> GSSHHHHHHSQDLENLYFQGSWKLLPENGSGSSENSGFSGSQINQVRPKLPLLKILHAAGAQGEMFTVKEVMHYLGQYIMVKQLYDQQEQHMVYCGGD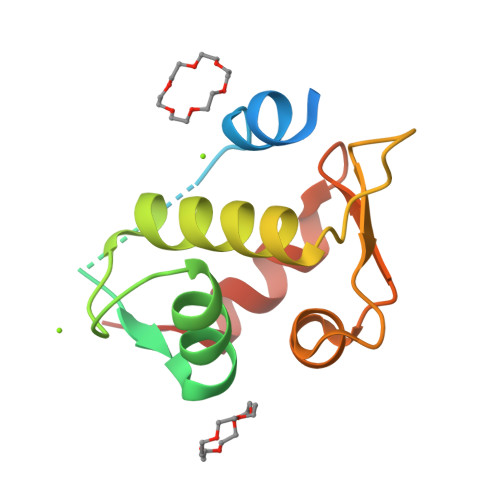LLGELLGRQSFSVKDPSPLYDMLRKNLVTLAT> MPNPSPPSSSSPVQTLISILRIIPDWSDRTQERGMRQHRTLYDHEKWMHHRSSYRHLRHLLSSLSSRVILSLIPPVIAFTLVAVVIASYNTAVALDLLPGIFPLLRSSSLPYQLTAPALALLLVFRTEASYSRFEEGRKSWTEVIAGANDFARQIISSVETSGDAQLKKALLQYIVAFPVALKCHVIYGSDIARDLQNLLEVDDLLVVLNSKHRPGCIIQFISRSLQLLKLEESRRIMLQSKISCFHEGIGICEQLIGTPIPLSYTRLTSRFLVLWHLTLPIILWDDCHWIVVPATFISAASLFCIEQVGVLIEEPFPMLALDDLCNSVRNNVQEALASEKLIRARLAAKGRIQSEQQFQNGQPRPENLYFQ

VCCN1 was recently identified as a voltage-gated chloride channel residing in the thylakoid membrane, where it plays a key role in photoreaction tuning to avoid the generation of reactive oxygen species (ROS). VCCN1 structurally resembles its animal homolog, bestrophin, a Ca2+-gated anion channel. However, unlike bestrophin channels, VCCN1 lacks the Ca2+-binding motif but instead contains an N-terminal charged helix that is anchored to the lipid membrane through an additional amphipathic helix. MdVCCN1 forms a symmetric homopentamer, with each subunit consisting of three domains: transmembrane domain (TMD), N-terminal domain (NTD), and stromal domain (SMD).

We then performed single-particle cryo-EM analyses of MdVCCN1 in detergent micelles (glyco-diosgenin; GDN), and in nanodiscs to investigate the structure in a native-like membrane environment. The structures were determined at 3.0 Å and 2.7 Å, respectively, with imposed C5 symmetry. Notably, the NAH is only visualized in the nanodisc structure and is disordered in the detergent micelles, indicating that the lipid environment is essential to stabilize this helix.>GSDELYRQSLEIISRYLREQATGAKDTKPMGRSGATSRKALETLRRVGDGVQRNHETAFQGMLRKLDIKNEDDVKSLSRVMIHVFSDGVTNWGRIVTLISFGAFVAKHLKTINQESCIEPLAESITDVLVRTKRDWLVKQRGWDGFVEFF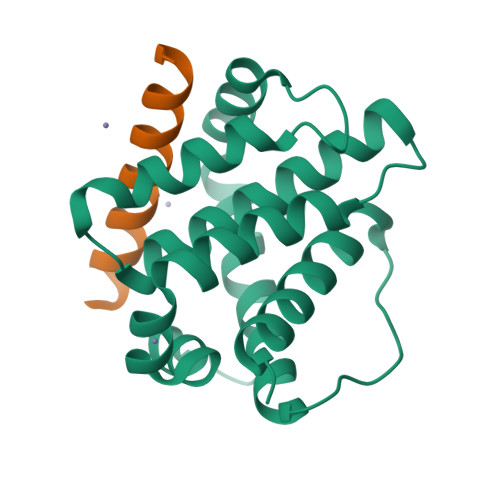HVEDL[2x];>XAPKEKEVAETLRKIGEEINEALKX[2x]>MTVESVNPETRAPAAPGAPELREPPVAGGGVPLLGHGWRLARDPLAFMSQLRDHGDVVRIKLGPKTVYAVTNPELTGALALNPDYHIAGPLWESLEGLLGKEGVATANGPLHRRQRRTIQPAFRLDAIPAYGPIMEEEAHALTERWQPGKTVDATSESFRVAVRVAARCLLRGQYMDERAERLCVALATVFRGMYRRMVVPLGPLYRLPLPANRRFNDALADLHLLVDEIIAERRASGQKPDDLLTALLEAKDDNGDPIGEQEIHDQVVAILTPGSETIASTIMWLLQALADHPEHADRIRDEVEAVTGGRPVAFEDVRKLRHTGNVIVEAMRLRPAVWVLTRRAVAESELGGYRIPAGADIIYSPYAIQRDPKSYDDNLEFDPDRWLPERAANVPKYAMKPFSAGKRKCPSDHFSMAQLTLITAALATKYRFEQVAGSNDAVRVGITLRPHD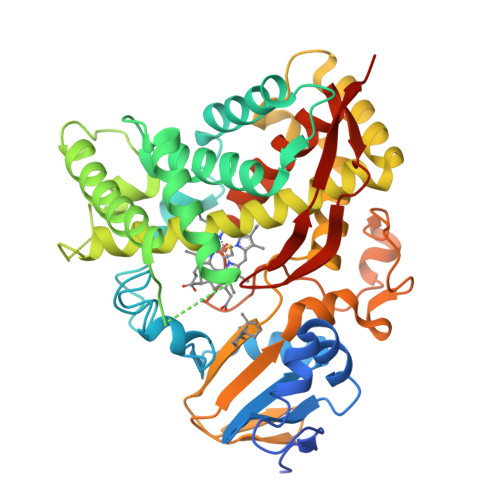LLVRPVARHHHHHH[2x]>[2x]GMTNNLKQRRIILDLAVTLDGFIEGKNGEVDWCIMDPDMGFTDFLNQ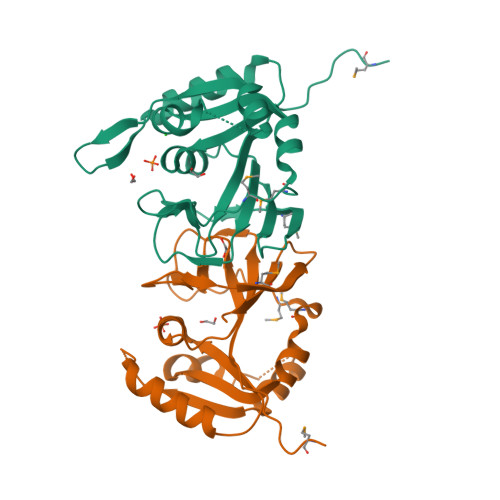IDTILYGRKSFDLWGQYIPKNEDPDTEKELWKLVHSKKKYVFSRTQNEIDNQAIFINDNILEEVNKLKKNPGKDIWLYGGASLITTFINLGLVDEFRLSIHPVVLGEGKPLFIDVKQRINLKMVNTRTFSSGVVQIVYHWNG>MSRRPTLRLGLDRDVYNIVLNLEQQGTDENGKRPRLTVDYVYDTIKRSNSSLARQKKRMLEDSIERVLAVRKEQAKAEEETDSDDLIEAQERERERQKAAQAQRDANLLNRQIAKSWGFASSPGAKAADGEKGTDTGSIATPAPATPAVAENMAADTPTTSTGPVLPASSTDRQPNGEPRPKKRKAAPKEIDRTPPTKVSILDIAGVDDTLQRLLKEVWFPLRGGEACEKMGYRYDNGVLLHGPSGCGKTTLAHAIAGSIGVAFIPVSAPSVIGGTSGESEKNIRDVFDEAIRLAPCLIFLDQIDAIAGRRESANKGMESRIVAEIMNGMDRIRQNTPLGKNVVVLAATNRPEFLDPAI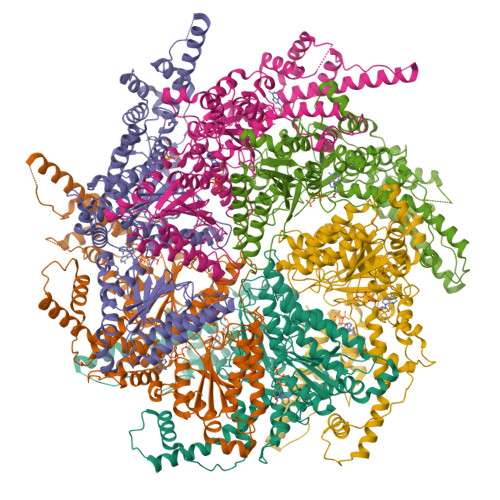RRRFSVEIDMGMPSERAREQILRSLTRDLSLADDINFKELAKMTPGYVGSDLQYVVKAAVSESFQANIDSLLAQARAKHPADHLANVSQPQRDWLLLEAHRDEEVSWPSTKITMEQFRKAVSLVQPASKREGFSTIPDTTWSHVGALEDVRKKLEMSIIGPIKNPELFTRVGIKPAAGILLWGPPGCGKTLVAKAVANESKANFISIKGPELLNKYVGESERAVRQLFSRAKSSAPCILFFDQMDALVPRRDDSLSDASARVVNTLLTELDGVGDRSGIYVIGATNRPDMIDEAIRRPGRLGTSIYVGLPSAEDRVKILKTLYRNTVKAPKKREGTNGEDVDMTDAAAEQQHQGTTDADLEKVALDLRCTGFSGADLGNLMQAAAQACLERVYTQRQQKRKEGGSVAEEEEIEPVITMEDWEKALNEVKPSVKDPEKYMHSGFAAALEHHHHHH[6x]> GQHTLKQFAADSALTTTTPLCSEVPL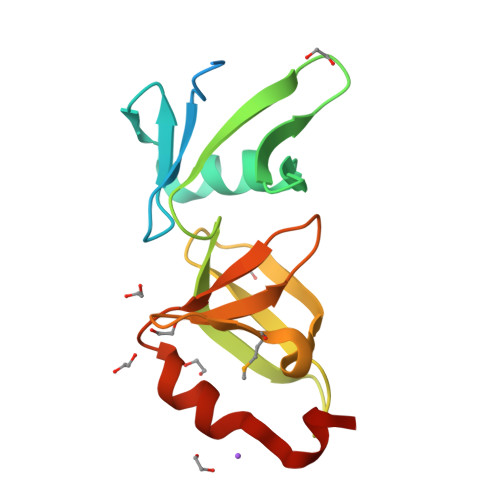FDINALGDWTYLGTSLPAKFAKLFASILHCIDDEYFLITPVEKVRVQVEDAPLLIVDFERAQPHSLLNVSTSIGTLHHNVDIKQMKLTDDSVYLPLERGLWGKLGRACYYNFVNEFNLSDLNEQ> HMSLSVANSTYETTALNSQKSSTDQPNSGSKSGQTLDLVNLGVAANFAILSKTGITDVYKSAITGDVGASPITGCAILLKCDEVTGTIFSVDACGPACKITDASRLTTAVGDMQIAYDNAAGRLNPDFLNLGAGTIGGKTLTPGLYKWTSTLNIPTDITISGSSTDVWIFQVAGNLNMSSAVRITLAGGAQAKNIFWQTAGAVTLGSTSHFEGNILSQTGINMKTAASINGRMMAQTAVTLQMNTVTIPQ

The FfIBP from Flavobacterium frigoris PS1 exhibits high TH activity and relatively strong recrystallization inhibition activity. The FfIBP structure is composed of parallel β-strands in a helical pattern, which is mainly stabilized by inner hydrophobic interactions and intramolecular hydrogen bonds with long α415. Additionally, the FfIBP has a capping head region that consists of two small turns and β-strands, which contain a disulfide bond. This disulfide bond increases the overall rigidity of the protein and reduces residual movement at the ice-binding site, thereby augmenting TH activity and protein stability.

The mutation site for FfIBP_CC1 was located in the top loop of the capping head region, which contained a largely flexible residue Gly121. Among these mutants, only FfIBP_CC1 and FfIBP_CC4 formed disulfide bonds within the intended area. However, FfIBP_CC1 did not exhibit any significant difference. Moreover, MD simulations using the FfIBP_CC1 structure indicated that the disulfide bond formation between C101 and C120 stabilized the fluctuation of residues in the capping head region. Consistent with our hypothesis, FfIBP_CC1, which has an additional disulfide bond on the capping head region, exhibited increased thermal stability, with a melting temperature (Tm) of 65 °C compared with wildtype FfIBP (60 °C). The TH activity of FfIBP_CC1 was akin to that of wild-type FfIBP at equivalent concentrations. The data indicated that FfIBP_CC1 significantly inhibited the growth of ice crystals, even at a low concentration of 0.4 µM, which is comparable to that of wildtype FfIBP. In addition, FfIBP_CC1 exhibited increased thermal stability, even when exposed to high concentrations of chemical denaturants such as DMSO, MeOH, Urea, propylene glycol, EtOH, and glycerol. Interestingly, unlike wildtype, FfIBP_CC1 underwent a two-step denaturation. Furthermore, the incorporation of disulfide bonds into the capping head region of FfIBP enhances its stability and resistance to thermal and chemical denaturation.2,4-dinitrophenyl 2-deoxy-2-fluoro-beta-D-glucopyranoside | C12 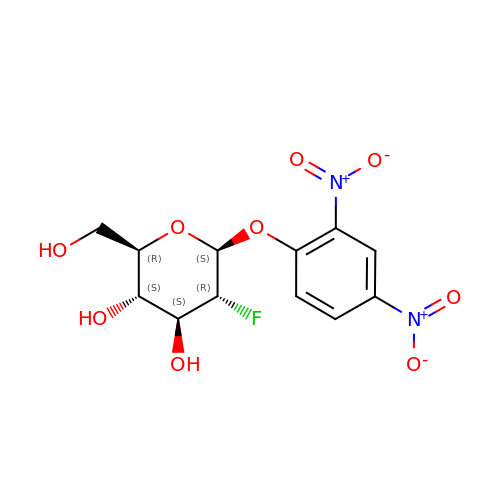H13 F N2 O9 | UFSBFVZQJZMIOU-LZQZFOIKSA-N> GEFTQSVSRLQSIVAGLKNAPSDQLINIFESCVRNPVENIMKILKGIGETFCQHYTQSTDEQPGSHIDFAVNRLKLAEILYYKILETVMVQETRRLHGMDMSVLLEQDIFHRSLMACCLEIVL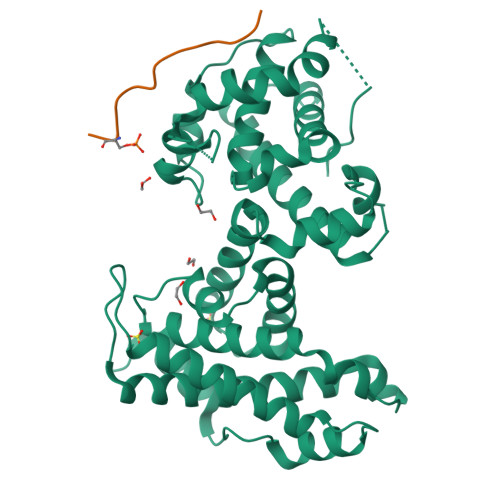FAYSSPRTFPWIIEVLNLQPFYFYKVIEVVIRSEEGLSRDMVKHLNSIEEQILESLAWSHDSALWEALQVSANKVPTCEEVIFPNNFETGRPKRTGSLALFYRKVYHLASVRLRDLCLKLDVSNELRRKIWTCFEFTLVHCPDLMKDRHLDQLLLCAFYIMAKVTKEERTFQEIMKSYRNQPQANSHVYRSVLLKSIKEERGDLIKFYNTIYVGRVKSFALKYDLANQDHMMDAPPLSPFPHIKQQ;> EASLLSFEKLDRASPDLWPE> MMQQRQVLMVEDTASVAALYKSYLNPLGLNVSIVGTGKEALSFIQDIIPDLILLDLRLPDMTGMEVLERVRKEHGNVPVVIMTAHGSIDIAVEAIRYGAQDFLIKPCEADRLRITVNKALKAESKSNTSTQSKQSDGAQYQGFIGNSLPMQAVYRVIESAASSKATVFITGESGTGKEVCAEAIHAASPRHDKPFIALNCAAIPKDLIESELFGHVKGAFTGASTERQGAVEMAHNGTLMLDELCEMDLDLQSKLLRFIQTGTYQKVGSSKMSSVDVRFVCATNRNPWEEVQEGRFREDLYYRLHVIPISLPPLRERGGDIIEIAHALLGLMSLEEGKSFSRFSEPVLRLFESYSWPGNVRELQNVIRNIVVLNTDDEVKLEMVPPPILEHHHHHH

Here, we use X-ray crystallography to study LuxO, the central quorum sensing regulator in Vibrio cholerae and related bacteria. LuxO belongs to the subfamily of AAA+ ATPases known as bacterial enhancer-binding proteins (bEBPs). In LuxO, as in NtrC proteins, the phosphorylation of an aspartate located within the R-domain activates the C domain for ATP hydrolysis and the opening/activation of σ54-dependent promoters. Here, we present crystal structures and in vitro and in vivo functional studies of LuxO that together reveal what is, to our knowledge, an entirely novel mechanism of AAA+ protein regulation, in which a regulatory segment of the protein prevents substrate ATP binding and hydrolysis by occupying a portion of the enzyme active site.

We determined the 1.6 Å resolution crystal structure of a V. angustum LuxO construct lacking the D domain but containing both R and C domains (denoted LuxO-RC). The structures of the individual R and C domain are very similar to those of homologs such as NtrC1 (root mean square [rms] deviations of 1.3 Å and 1.7 Å, respectively), although the relative positioning of the R and C domains is unique. Rather than forming closed rings, V. angustum LuxO monomers in the crystals form continuous helical arrays with six subunits per turn. In the V. angustum LuxO-RC structure, the R domain is nestled between the two lobes of the C domain, forming a discrete interface with each. Interface I is dominated by an interaction between α-helix 5 (α5) of the R domain and α7 of the C domain. In interface II, α4 and β-strand 5 (β5) of the R domain interact with α13 of the C domain. The R and C domains are connected by a 20-residue linker (denoted R-C linker, residues 123–142). Strikingly, residues 137–142 of the R-C linker occupy a substantial portion of the C domain active site, sterically occluding the binding of the ATP substrate. The R-C linker is stabilized in the active site by an extensive network of H-bonds, including four with residues within the R domain and three with residues within the C domain. Gly 141 of the R-C linker appears to be especially important, as it not only makes three key H-bonds using its main chain nitrogen and oxygen atoms but also occupies a position deep within the active site that could not accommodate a larger residue.> MSYASRTLGPMQTSSDRHEYPAHWEADVVLRDGGTARVRPITVDDAERLVSFYEQVSDESKYYRFFAPYPRLCAKDVHRFTHHDFVDRVGLAATIGGEFIATVRYDRIGAGGTPATA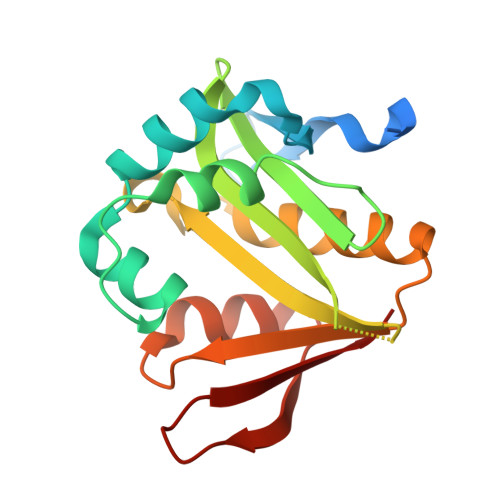PADEAEVAFLVQDAHQGRGVASALLEHIAAVARERGIRRFAAEVLPANNKMIKVFMDAGYTQKRSFEDGVVRLEFDL> MSLKEIGPNSLLLEDSHSLSQLLKKNYRWYSPIFSPRNVPRFADVSSITESPETLKAIRDFLVERYRTMSPAPTHILGFDARG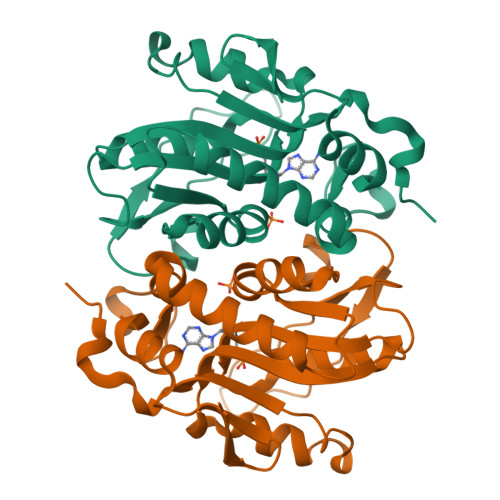FLFGPMIAVELGIPFVLMRKADKNAGLLIRSEPYEKEYKEAAPEVMTIRHGSIGKNSRVVLIDDVLATGGTALSGLQLVEASGAEVVEMVSILTIPFLKAAERIHSTAGGRYKNVRFIGLLSEDVLTEANCGDLNDYTGPRVLSCSDLLVNQ>[4x]MKTVTVKNLIIGEGMPKIIVSLMGRDINSVKAEALAYREATFDILEWRVDHFMDIASTQSVLTAARVIRDAMPDIPLLFTFRSAKEGGEQTITTQHYLTLNRAAIDSGLVDMIDLELFTGDADVKATVDYAHAHNVYVVMSNHDFHQTPSAEEMVSRLRKMQALGADIPKIAVMPQSKHDVLTLLTATLEMQQHYADRPVITMSMAKEGVISRLAGEVFGSAATFGAVKQASAPGQIAVNDLRSVLM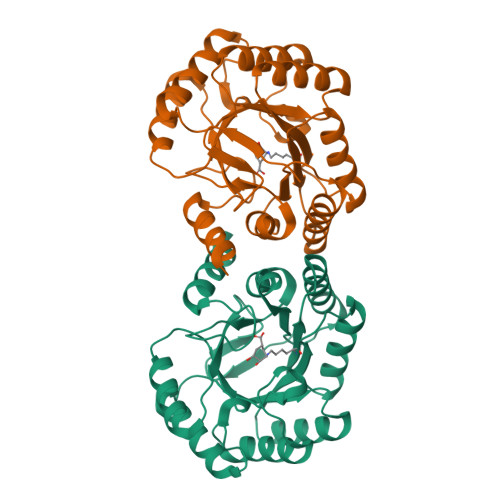ILHNA>MPNSLDVHQRQTRSNVSTPTLRPRDDTASSFVSKDPGANVRVVVRVRAFLPRELERNAECIVEMDPATERTSLLVPQETDFADARGARSRRVLEEKSFTFDKSFWSHNTEDEHYATQEHVYDSLGEEFLDHNFEGYHTCIFAYGQTGSGKSYTMMGTPDQPGLIPRTCEDLFQRIASAQDETPNISYNVKVSYFEVYNEHVRDLLAPVVPNKPPYYLKVRESPTEGPYVKDLTEVPVRGLEEIIRWMRIGDGSRTVASTKMNDTSSRSHAVF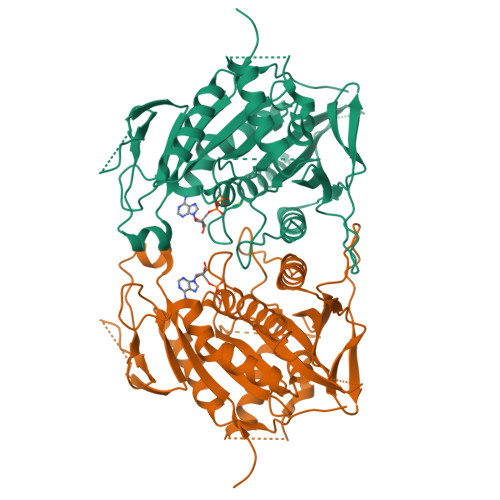TIMLKQIHHDLETDDTTERSSRIRLVDLAGSERAKSTEATGQRLREGSNINKSLTTLGRVIAALADPKSSASRPSSPVKSGRGRTPGPANSVVPYRDSVLTWLLKDSLGGNSKTAMIACISPTDYDETLSTLRYADQAKRIRTRAVVNQVDGVSAAERDAQIPSIVHRKCF[4x]> MTEMELKLIKIDTSHYFEKKPGLGERVDYAGRCFYNKFQRVNAMLTSSLIQKHLKREIEIAHNLILRND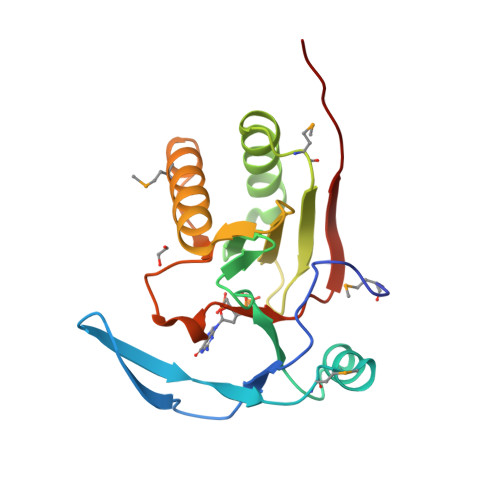KVENIVFDYNGRNPERFYHKAQLLLREEGFMNFTAYNTKTPGHLHLYVHKGHTELGEGERLVKTLSMKLAQGLPKEWKVFPSNEWPKEFNILALPYEVFAKERGSSWAKHL> GAMAVYPCGICTNEVNDDQDAILCE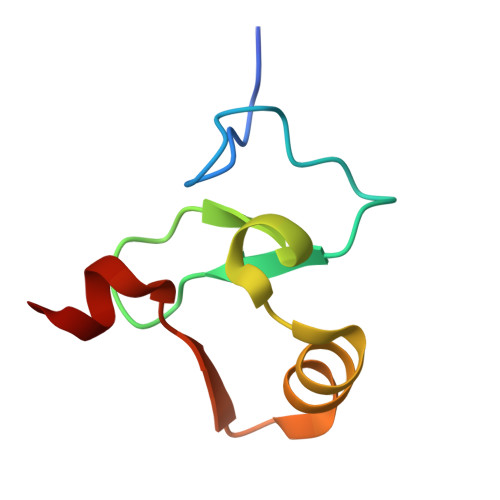ASCQKWFHRICTGMTETAYGLLTAEASAVWGCDTCMAD> MKILVA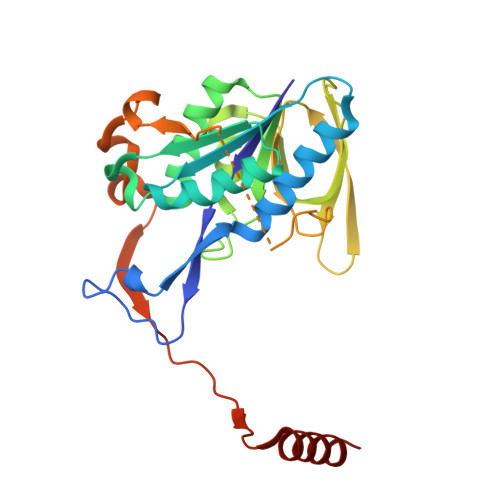VKQTAALEEDFEIREDGMDVDEDFMMYDLNEWDDFSLEEAMKIKESSDTDVEVVVVSVGPDRVDESLRKCLAKGADRAVRVWDDAAEGSDAIVVGRILTEVIKKEAPDMVFAGVQSSDQAYASTGISVASYLNWPHAAVVADLQYKPGDNKAVIRRELEGGMLQEVEINCPAVLTIQLGINKPRYASLRGIKQAATKPIEEVSLADIGLSANDVGAAQSMSRVRRMYIPEKGRATMIEGTISEQAAKIIQIINEFKGA> MNDSILLGLIGQGLDLSRTPAMHEAEGLAQGRATVYRRIDTLGSRASGQDLKTLLDAALYLGFNGLNITHPYKQAVLPLLDEVSEQATQLGAVNTVVIDATGHTTGHNTDVSGFGRGMEEGLPNAKLDSVVQVGAGGVGNAVAYALVTHGVQKLQVADLDTSRAQALADVINNAVGREAVVGVDARGIEDVIAAADGVVNATPMGMPAHPGTAFDVSCLTKDHWVGDVVYMPIETELLKAARALGCETLDGTRMAIHQAVDAFRLFTGL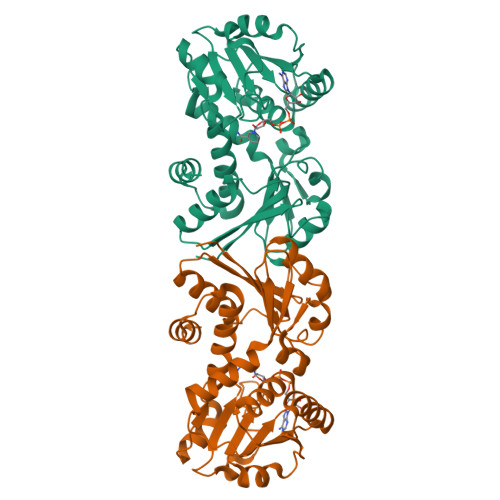EPDVSRMRETFLSL4-fluorobenzene-1,2-diol | C6 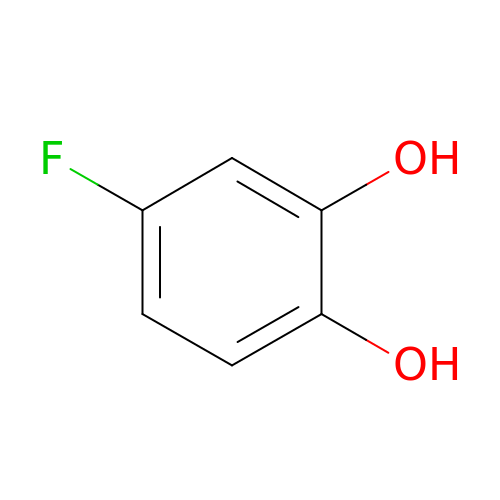H5 F O2 | NFWGQJUHSAGJBE-UHFFFAOYSA-N> M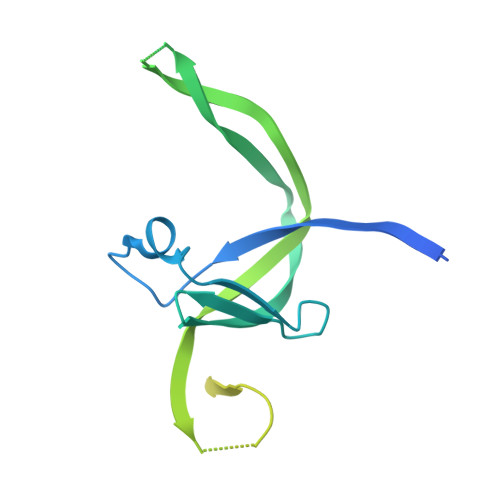AAAADERSPEDGEDEEEEEQLVLVELSGIIDSDFLSKCENKCKVLGIDTERPILQVDSCVFAGEYEDTLGTCVIFEENVEHADTEGNNKTVLKYKCHTMKKLSMTRTLLTEKKEGEENIGGVEWLQIKDNDFSYRPNMICNFLHENEDEEVVASAPDKSLELEEEEIQMNDSSNLSCEQEKPMHLEIEDSGPLIDIPSETEGSVFMETQMLP> EFLADSSAHLDLRNFYQLRDYRQHDAPQSQAGNWSQGFVLRLQSGFTGGPLGFGLDATGLLGVKLDSGRGRSNDGTLPFGANSKEPVDDYSHLGLTAKLRYSQTQLQVGILMPQLPVAFRDDVRLLPQTFDGALLTSSEIEGLTLTAGQLWKSRTRESAGSDDMYIMGRDKAHASDEFNLAGATYAFTPRLSASYYYGQLKDIYRQHYLGLLHTLPLGEGLSLRSDLRYFDSGEDGAAISGPVDNRNLNAMLTLRAGAHAFGIGVQKMIGNDAFPVLNGYTTPYVANLMAYQTFTRPQEKSWQLRYDYDFAGLGLPGLNLMTRYVQGRDIDRGAGRADDSEWERNTDLSYVIQSGPLKSVALKWRNITYRSRYGADLDENRFIVNYTLKLWGGHHHHHH

In such microorganisms, the majority of small molecules are taken up by members of the OprD outer membrane protein family. Here we show that OprD channels require a carboxyl group in the substrate for efficient transport, and based on this we have renamed the family Occ, for outer membrane carboxylate channels. As expected from pairwise sequence identities that range from 35%–50%, the Occ proteins share a similar architecture, with a slightly off-center constriction formed by the inward-folded extracellular loops L3 and L7 and residues in the barrel wall. The transport data demonstrate that Occ channels have a pronounced preference for substrates with a carboxyl group, due to the universal presence of a basic ladder on one side of the barrel wall.

To determine if the phylogenetic subdivision of Occ proteins exists at the structural level, we determined X-ray crystal structures for seven Occ family members (OccD2, OccD3, and OccK2–K6). The pores of the proteins within the OccK subfamily show a considerable variation in size and shape, suggesting differences in substrate preferences within subfamilies as well. For OccK channels, conductance values are on average somewhat larger than those of OccD subfamily members, ranging from ∼50 pS for OccK4 to ∼300 pS for OccK1, OccK5, and OccK7. OccK4 was indeed the most efficient phenylacetate uptake channel of the proteins tested; however, the specific activities are very low and, as for vanillate, high substrate concentrations had to be used. Thus, phenylacetate is not a preferred substrate for any of the tested channels.Here, we describe the biochemical analysis of these two proteins and show that the enzyme encoded by HS5.18 catalyzes the formation of cytidine diphosphate (CDP)-6-d-fructose from cytidine triphosphate (CTP) and d-fructose-6-phosphate, and the enzyme encoded by HS5.17 reduces CDP-6-d-fructose with NADPH to generate CDP-6-d-glucitol. The overall fold of this enzyme places it into the well-characterized short-chain dehydrogenase/reductase (SDR) superfamily of enzymes. Unique to this protein is an extended α-helix that precedes the beginning of the Rossmann fold that is found in all SDR proteins. The individual subunits adopt a bilobal-type architecture with the N-terminal domain composed of Met 1 to Thr 201 and the C-terminal domain formed by Ala 202 to Glu 332.

The second structure of the oxidoreductase reported here was solved at 2.2 Å resolution and refined to an overall R-factor of 21.1%. The asymmetric unit also contained a dimer, and the α-carbons for the two subunits superimpose with a root-mean-square deviation of 0.4 Å. Whereas the enzyme was crystallized in the presence of CDP-6-d-glucitol and NADP(H), no electron density was observed for the dinucleotide. The electron density was unambiguous for the CDP-6-d-glucitol ligands in both subunits, however, as can be seen in Figure 8a for the ligand bound to Subunit B. The α-carbons for Subunit B with either bound CDP or CDP-6-d-glucitol correspond with a root-mean-square deviation of 0.5 Å. The glucitol C1′ hydroxyl lies within 3.2 Å of the guanidinium group of Arg 208. The C2′ hydroxyl hydrogen bonds with the backbone carbonyl oxygen of Thr 195. The C3′ and C4′ hydroxyls are bridged by Nε2 of Gln 196, and the C5′ hydroxyl hydrogen bonds to the side chain of Glu 140. Although the NADP(H) ligand was not bound, it is possible to approximate the position of the dinucleotide by superimposing the two structures presented here. This superposition suggests that the C2′ carbon of the substrate is within 3 Å of C4 of the nicotinamide ring of the cofactor and lies on the si face. In addition, the model of the enzyme with bound CDP-6-d-glucitol represents the first molecular view of the manner in which an enzyme in this superfamily can accommodate an open-chain nucleotide-linked sugar in its active site pocket.

>[2x]MGSSHHHHHHSSGENLYFQGHMNEILKKRLKLLKNNFGTHINKIANKKILITGANGYIGSILTLILHGNAKLYCLVRNKDKMIDRFQEICGDIDKIDIYEDLYKIQDKIDIVIHCAAPTQSDFFIENPIDTVDIIYTNTKNILDFSKKNNVEKIIFLSTMEIYGDVIGDNIVEDDIGKFSVTNIRNSYPLAKQISEFMVHSYSKKYSLSTAIVRLTQAIGPTAQINDNRVYMDFIRSAIKKSQITLFTKGETKREYIDVFDVATAIIFVMCEKKMFEIYNISNPNIFISIYDLAKTISAKLNVQVVFDLQRDTSQYLPSFSRRLNSKKIYQLGWTPLFDLNQSLDDMIKYIKEVNE>GKKKVCYYYDGDIGNYYYGQGHPMKPHRIRMTHNLLLNYGLYRKMEIYRPHK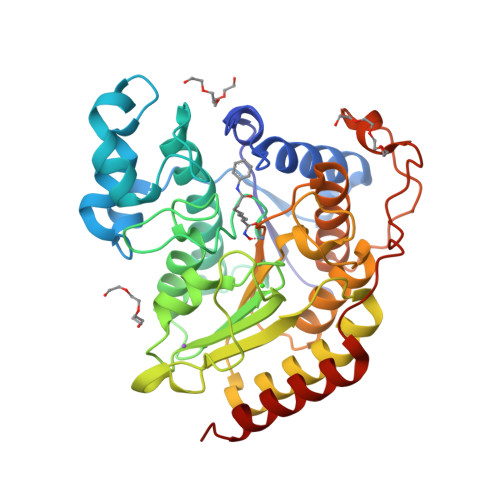ATAEEMTKYHSDEYIKFLRSIRPDNMSEYSKQMQRFNVGEDCPVFDGLFEFCQLSTGGSVAGAVKLNRQQTDMAVNWAGGLHHAKKSEASGFCYVNDIVLAILELLKYHQRVLYIDIDIHHGDGVEEAFYTTDRVMTVSFHKYGEYFPGTGDLRDIGAGKGKYYAVNFPMRDGIDDESYGQIFKPIISKVMEMYQPSAVVLQCGADSLSGDRLGCFNLTVKGHAKCVEVVKTFNLPLLMLGGGGYTIRNVARCWTYETAVALDCEIPNELPYNDYFEYFGPDFKLHISPSNMTNQNTPEYMEKIKQRLFENLRMLPH[3x]>MHHHHHHPEIVDTCSLASPASVCRTKHLHLRCSVDFTRRTLTGTAALTVQSQEDNLRSLVLDTKDLTIEKVVINGQEVKYALGERQSYKGSPMEISLPIALSKNQEIVIEISFETSPKSSALQWLTPEQTSGKEHPYLFSQCQAIHCRAILPCQDTPSVKLTYTAEVSVPKELVALMSAIRDGET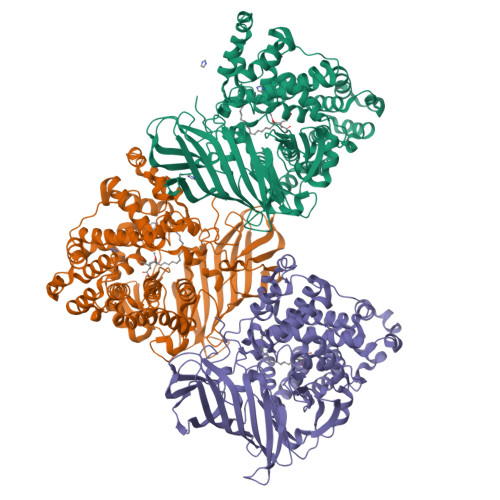PDPEDPSRKIYKFIQKVPIPCYLIALVVGALESRQIGPRTLVWSEKEQVEKSAYEFSETESMLKIAEDLGGPYVWGQYDLLVLPPSFPYGGMANPCLTFVTPTLLAGDKSLSNVIAHEISHSWTGNLVTNKTWDHFWLNEGHTVYLERHICGRLFGEKFRHFNALGGWGELQNSVKTFGETHPFTKLVVDLTDIDPDVAYSSVPYEKGFALLFYLEQLLGGPEIFLGFLKAYVEKFSYKSITTDDWKDFLYSYFKDKVDVLNQVDWNAWLYSPGLPPIKPNYDMTLTNACIALSQRWITAKEDDLNSFNATDLKDLSSHQLNEFLAQTLQRAPLPLGHIKRMQEVYNFNAINNSEIRFRWLRLCIQSKWEDAIPLALKMATEQGRMKFTRPLFKDLAAFDKSHDQAVRTYQEHKASMHPVTAMLVGKDLKVD[3x]>EDADKLPHTKVTLVAPPQVHPHEQATKSGPKVVEFTMTIEEKKMVIDDKGTTLQAMTFNGSMPGPTLVVHEGDYVQLTLVNPATNAMPHSVDFHGATGALGGAKLTNVNPGEQATLRFKADRSGTFVYHCAPEGMVPWHVVSGMSGTLMVLPRDGLKDPQGKPLHYDRAYTIGEFDLYIPKGPDGKYKDYATLAESYGDTVQVMRTLTPSHIVFNGKVGALTGANALTAKVGETVLLIHSQANRDTRPHLIGGHGDWVW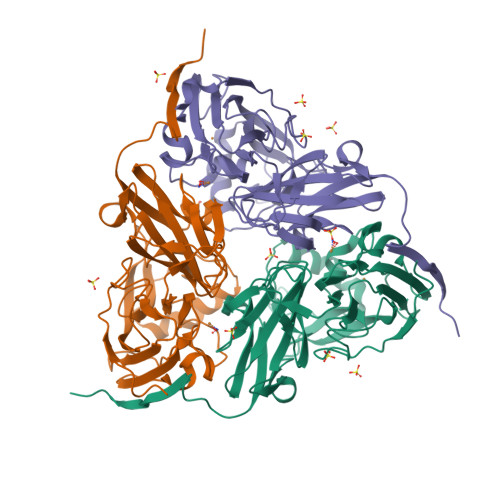ETGKFANPPQRDLETWFIRGGSAGAALYTFKQPGVYAYLNHNLIEAFELGAAGHIKVEGKWNDDLMKQIKAPAPIPR[6x]>[2x]MNTPEHMTAVVQRYVAALNAGDLDGIVALFAD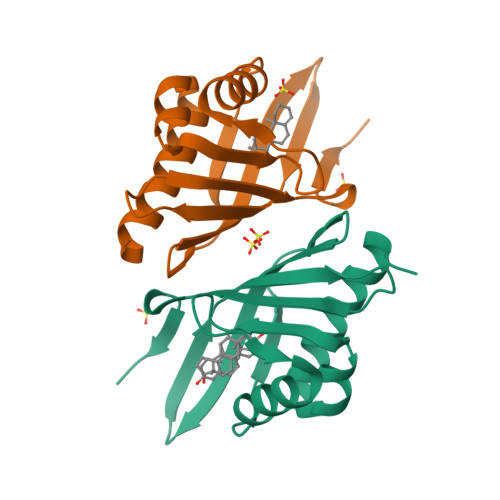DATVENPVGSEPRSGTAAIREFYANSLKLPLAVELTQEVRAVANEAAFAFTVSFEYQGRKTVVAPINHFRFNGAGKVVSMRALFGEKNIHAGA> ADPMIAEELLRAGRLDDALKALQEQVRSQPSNATLRIFLFQLLAVMGQWARAQNQLKVVGELDASALPMVQTYSTAIDCEALRREVFAGRLTPVILGQPAEWIAPLLQALSLDAEGHGEAAQALREQAFDAAPAVPGRIGEA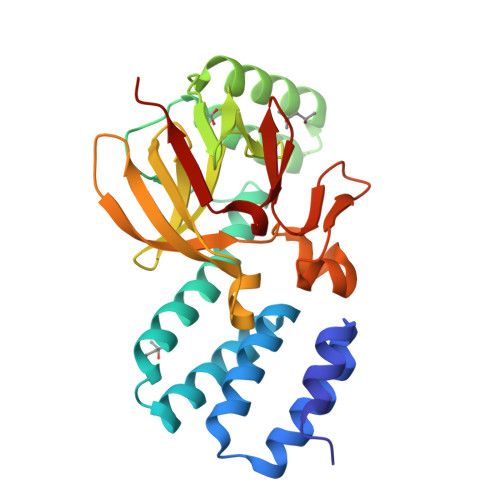PFAWLADADTRLGPVLEVIVNGRYAWLPMSNLRSLKVEAPSDLRDLVWLPAELTLANGGATVALLPARYAETVEHGDDAARLGRKTEWLDSGLPVGQRLFVTDAGETALFDLRELDFEPTDA2-{2-[4-(1,1,3,3-TETRAMETHYLBUTYL)PHENOXY]ETHOXY}ETHANOL 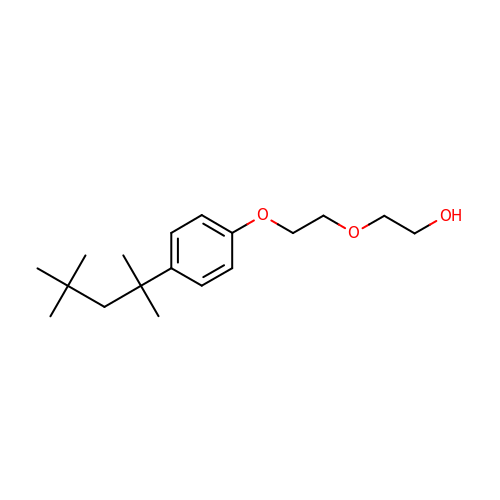| C18 H30 O3 | LBCZOTMMGHGTPH-UHFFFAOYSA-N>[3x]MGFLDGKRILLTGLLSNRSIAYGIAKACKREGAELAFTYVGDRFKDRITEFAAEFGSELVFPCDVADDAQIDALFASLKTHWDSLDGLVHSIGFAPREAIAGDFLDGLTRENFRIAHDISAYSFPALAKAALPMLSDDASLLTLSYLGAERAIPNYNTMGLAKAALEASVRYLAVSLGAKGVRVNAISAGPIKTLAASGIKSFGKILDFVESNSPLKRNVTIEQVGNAGAFLLSDLASGVT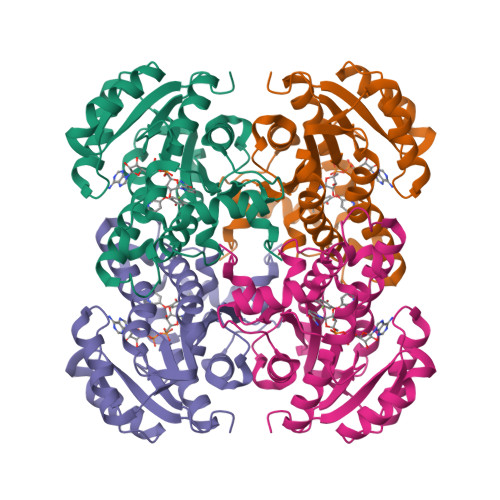AEVMHVDSGFNAVVGGMAGLEEKLAAALEHHHHHH> MKFIIEALKRVRERRPLVHNITNFVVMNTTANALLALGASPVMAHAEEELEEMIRLADAVVINIGTLDSGWRRSMVKATEIANELGKPIVLDPVGAGATKFRTRVSLEILSRGVDVLKGNFGEISALLGEEGKTRGVDSLEYGEEEAKKLTMNAAREFNTTVAVTGAVDYVSDGR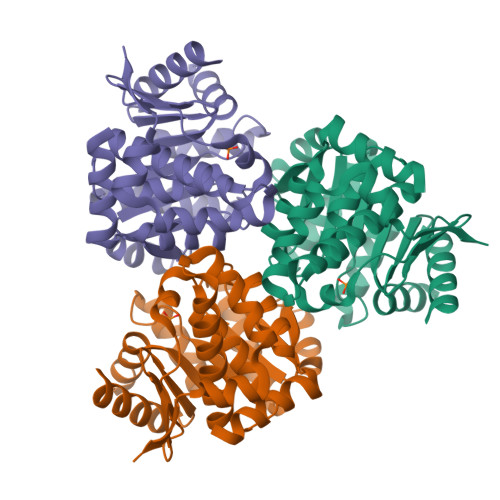RTFAVYNGHELLGRVTGTGCMVAALTGAFVAVTEPLKATTSALVTFGIAAEKAYEEAKYPGSFHVKLYDWLYRINENVIRTYAKVREVEL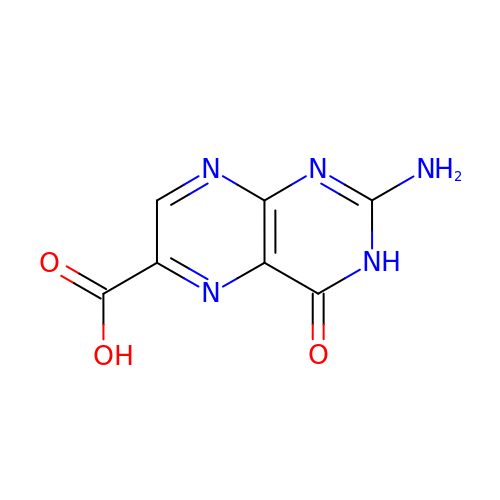6-CARBOXYPTERIN | C7 H5 N5 O3 | QABAUCFGPWONOG-UHFFFAOYSA-N>MGHHHHHHMATLICGSIAYDNIMTFEGRFREHILPDQVHLINLSFLVPTMRREFGGCAGNIAYALNLLGGDARMMGTLGAVDAQPYLDRMDALGLSREYVRVLPDTYSAQAMITTDLDNNQITAFH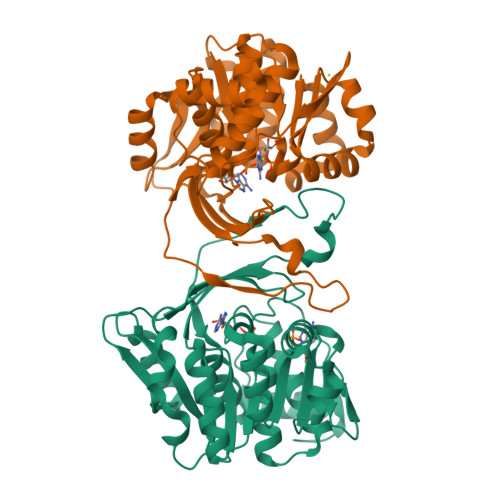PGAMMQSHVNHAGEAKDIKLAIVGPDGFQGMVQHTEELAQAGVPFIFDPGQGLPLFDGATLRRSIELATYIAVNDYEAKLVCDKTGWSEDEIASRVQALIITRGEHGATIRHRDGTEQIPAVRAERVIDPTGCGDAFRGGLLYGIEHGFDWATAGRLASLMGALKIAHQGPQTYAPTRAEIDARFETAFGYRPK[6x]4-BUTYL-1,2-DIPHENYL-PYRAZOLIDINE-3,5-DIONE 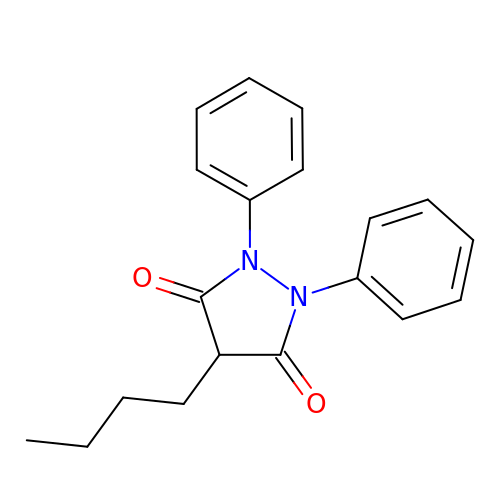| C19 H20 N2 O2 | VYMDGNCVAMGZFE-UHFFFAOYSA-N>[2x]GMASDEGKLFVGGLSFDTNEQSL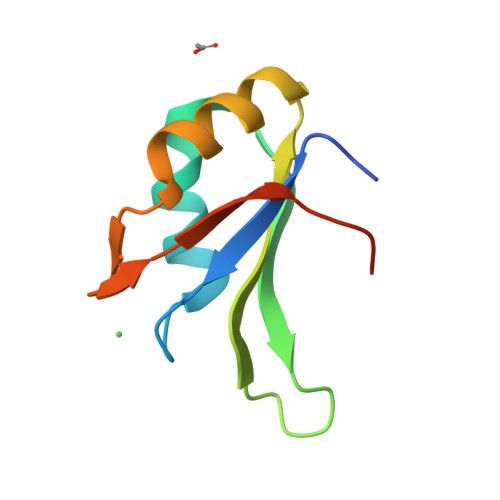EQVFSKYGQISEVVVVKDRETQRSRGFGFVTFENIDDAKDAMMAMNGKSVDGRQIRVDQAGKSSDNRSR> SSNSRFRHRKISVKQHLKIYLPNDLKHLDKDELQQREVVEIETGVEKNEEKEVHLHRILQMGSGHTKHKDYIPTPDASMTWNEYDKFYTGSFQETTSYIKFSATVEDCCGTNYNMDERDETFLNEQVNKGSSDILTEDEFEILCSSFEHAIHERQPFLSMDPESILSFEELKPTLIKSDMADFNLRNQLNHEINSHKTHFITQFDPVSQMNTRPLIQLIEKFGSKIYDYWRERKIEVNGYEIFPQLKFERPGEKEEIDPYVCFRRREVRHPRKTRRIDILNSQRLRALHQELKNAKDLALLVAK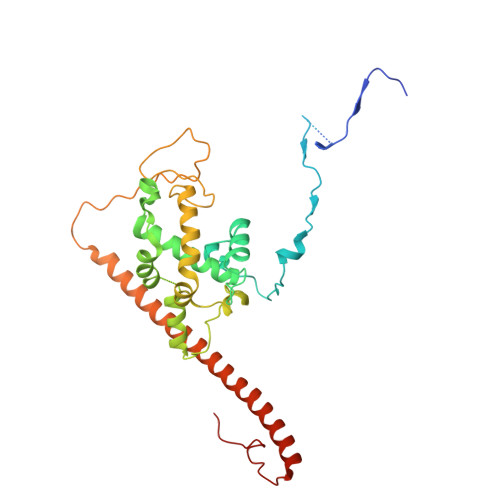RENVSLNWINDELKIFDQRVKIKNLKRSLNISGEDDDLINHKRKRPT>[2x]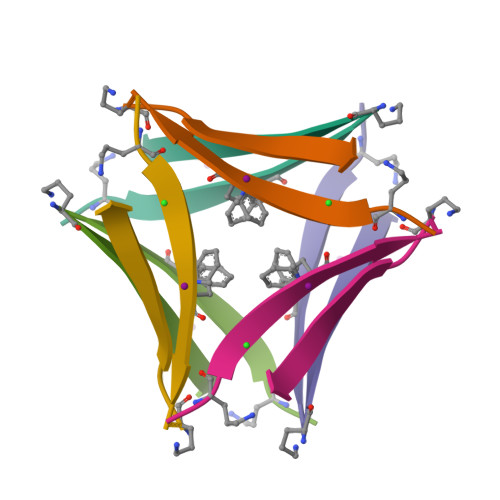HAKLVFFAEAAIIGLMV>VGSLNCIVAVSQNMGIGKNGDLPWPPLRNEFRYFQRMTTTSSVEGKQNLVIMGKKTWFSIPEKNRPLKGRINLVLSRELKEPPQGAHFLSRSLDDALKLTEQPELANKVDMVWIVGGSSVYKEAMNHPGHLKLFVTRIMQDFESDTFFPEIDLEKYKLLPEYPGVL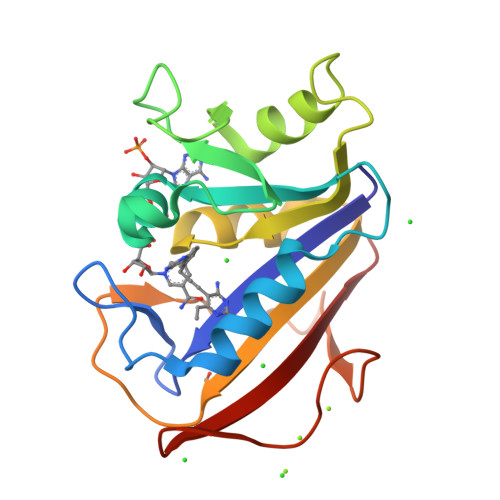SDVQEEKGIKYKFEVYEKND[2x]> ASEIELVF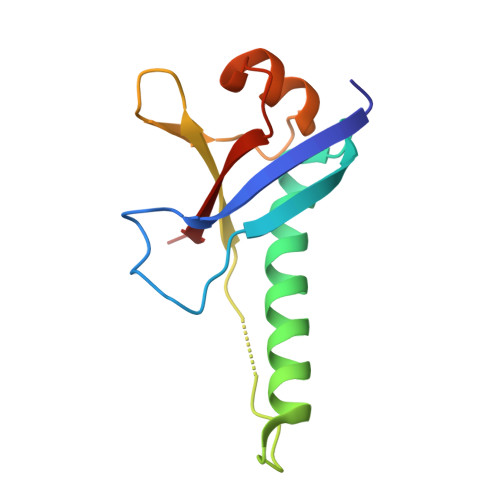RPHPTLMEKDDSAQTRYIKTSGNATVDHLSKYLAVRLALEELRSKGESNQMNLDTASEKQYTIYIATASGQFTVLDGSFSLELVSEKYWKVNKPMELYYAPTK>GSMGNYMGNPWTEYMAKYDIEEVHGSGIRVDLGEDAEVAGTQYRLPSGKCPVFGKGIIIENSKTTFLTPVATGNQYLKDGGFAFPPTEPLMSPMTLDDMRLLYKDNEDVKNLDELTLCSRHAGNMIPDNDKNSNYKYPAVYDDKDKKCHILYIAAQENNGPRYCNKDESKRNSMFCFRPAKDISFQNLVYLSKNVVHNWEKVCPRKNLQNAKFGLWVDGNCEDIPHVNEFSANDLFECNKLVFELSASDQPKQYEQHLTQQAKDIGAGPVASCFTTRMSPPQQICLNSVVNTALSGGSGGGNAAMIKSAFLPTGAFKADRYKSHGKGYNWGNYNTETQKCEIFNVKPTCLINDKNYIATTALSHPIEVEAAA[2x]

Invasion of human erythrocytes by Plasmodium falciparum (Pf) merozoites relies on the interaction between two parasite proteins: apical membrane antigen 1 (AMA1) and rhoptry neck protein 2 (RON2). AMA1 is comprised of three domains with domains 1 and 2 together forming a hydrophobic groove, the binding site for RON2L. Immunization with AMA1 bound to RON2L, a 49-amino acid peptide from its ligand RON2, has shown superior protection by increasing the proportion of neutralizing antibodies. To advance vaccine development, here we engineered chimeric antigens by replacing the AMA1 DII loop, displaced upon ligand binding, with RON2L.

A fusion chimera engineered using the HP41 AMA1 sequence was ultimately selected for structural studies based on yield and stability of the recombinant protein. The structure of the Fusion-FD12 protein incorporating residues 105 (2nd residue in the chimera) through 470 including the inserted PfRON2L sequence was determined to 1.55 Å resolution. Clear, contiguous electron density in the apical groove of Fusion-FD12 enabled unambiguous tracing of the entire PfRON2L sequence. Structural analysis revealed that the Fusion-FD12 protein adopts a conserved architecture relative to the structure of the previously observed binary complex20 with a root mean square deviation (rmsd) of 0.61 Å over 252 Cα positions. Moreover, RON2L in the fusion and binary complex overlay with an rmsd of 0.53 Å over 34 Cα positions. The core interactions between RON2L and AMA1 are retained in Fusion-FD12 including R376 of PfRON2L (R2041 in PfRON2) that docks into a pocket at the end of the PfAMA1 apical groove, and P368 (P2033 in PfRON2) that docks into a pocket formed by Y142, Y234, and Y236. Overall, all the AMA1 loops (1b, c, d, and f) that pack against the C-terminal end of the RON2L sequence are highly conserved (rmsd of 0.21 Å over 76 Cα positions) relative to the binary complex. In contrast, some differences are observed in loops 1e/1a that pack against the N-terminal section of the RON2 sequence. Notably, the sidechain of E136 on loop 1a is displaced by 2.5 Å and no longer forms a hydrogen bond with the sidechain of N233 positioned on loop 1e (Fig. 2E-Box 1). The loss of the hydrogen bond may also be responsible for the observed loop displacements, though it should be noted that differences in crystal packing between the fusion structure presented herein and the binary PfAMA1-RON2 structure may also contribute to observed shifts. Furthermore, many of the sidechains on loop 1e adopt different rotameric states with N228, N231 and D229 showing relatively similar displacement (~2.9 Å, 3.1 Å, and 3.4 Å) while K230 (~7.2 Å) and S232 (~6.9 Å) show significantly larger shifts (Fig. 2E-Box 2), which may alter epitopes in loop 1e.>[3x]MAELT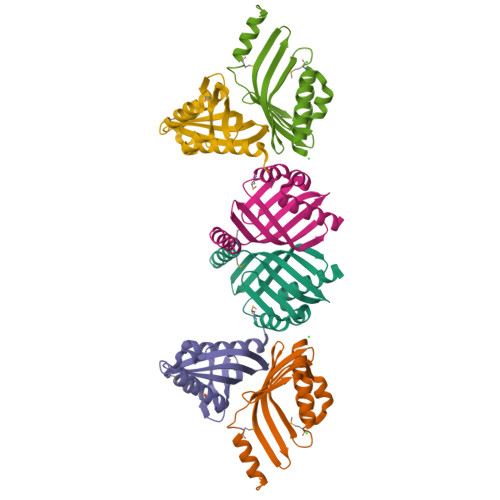ETSPETPETTEAIRAVEAFLNALQNEDFDTVDAALGDDLVYENVGFSRIRGGRRTATLLRRMQGRVGFEVKIHRIGADGAAVLTERTDALIIGPLRVQFWVCGVFEVDDGRITLWRDYFDVYDMFKGLLRGLVALVVPSLKATL> MVVMVMMFKILRKERLAPGINLFEIESPRIAKHAKPGQFVMIRLHEKGERIPLTIADVDISKGSITIVAQEVGKTTRELGTYEAGDYILDVLGPLGKPSHIDYFGTVVMIGGGVGVAEIYPVAKAMKEKGNYVISILGFRTKDLVF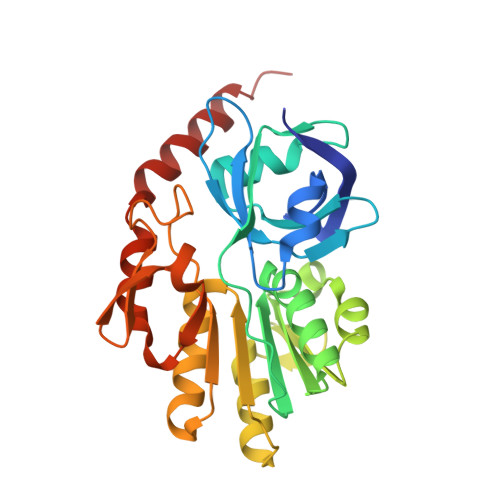WEDKLRSVSDEVIVTTNDGSYGMKGFTTHALQKLIEEGRKIDLVHAVGPAIMMKAVAELTKPYGIKTVASLNPIMVDGTGMCGACRVTVGGEVKFACVDGPEFDAHLVDWDQLMNRLAYYRDLEKISLEKWERERRMV>[2x]HHHLGNKLSISDLKDIKNKKVLVRVDFNVPIENGIIKDTNRITATLPTINHLKKEGASKIILISHCGRPDGLRNEKYTLKPVAETLKGLLGEEVLFLNDC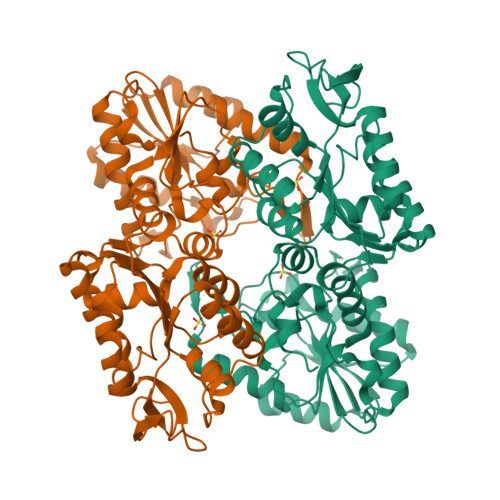VGKEVEDKINAAKENSVILLENLRFHIEEEGKGVDANGNKVKANKEDVEKFQNDLTKLADVFINDAFGTAHRAHSSMVGVKLNVKASGFLMKKELEYFSKALENPQRPLLAILGGAKVSDKIQLIKNLLDKVDRMIIGGGMAYTFKKVLNNMKIGTSLFDEAGSKIVGEIMEKAKAKNVQIFLPVDFKIADNFDNNANTKFVTDEEGIPDNWMGLDAGPKSIENYKDVILTSKTVIWNGPQGVFEMPNFAKGSIECLNLVVEVTKKGAITIVGGGDTASLVEQQNKKNEISHVSTGGGASLELLEGKELPGVLALSN>[2x]MTFERNKTLYWGGALWSPPSNWNPFTPWNAVAGTIGLVYEPLFLYDPLNDKFEPWLAEKGEWVSNNEYVLTLRKGLRWQDGVPLTADDVVFTFEIAKKYTGISYSPVWNWLGRIERVDERTLKFVFSDPRYQEWKQMLINTPIVPKHIWENKTEEEVLQAANENPVGSGPYYVESWADDRCVFKKNGNWWGIRELGYDPKPERIVELRVLSNNVAVGMLMKGELDWSNFFLPGVPVLKKAYGIVTWYENAPYMLPANTAGIYINVNKYPLSIPEFRRAMAYAINPEKIVTRAYENMVTAANPAGILPLPGYMKYYPKEVVDKYGFKYDPEMAKKILDELGFKDVNKDGFREDPNGKPFKLTIECPYGWTDWMVSIQSIAEDLVKVGINVEPKYPDYSKYADDLYGGKFDLILNNFTTGVSATIWSYFNGVFYPDAVESEYSYSGNFGKYANPEVETLLDELNRSNDDAKIKEVVAKLSEILLK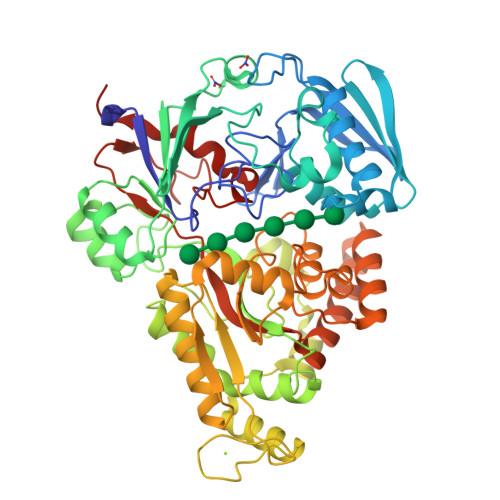DLPFIPLWYNGAWFQASEAVWTNWPTEKNPYAVPIGWNGWWQLTGIKTLFGIEAKHHHHHH> ALKRKIEAAKMPKDAREKTEAELQKLKMMSPMSAEATVVRGYIDWMLQVPWNSRSKVKKDLVKAQEVLDTDHYGLERVKDRILEYLAVQSRVSKIKGPILCLVGPPGVGKTSLGQSIAKATGRQYVRMALGGVRDEAEIRGHRRTYIGSMPGKLIQKMAKVGVKNPLFLLDQIDKMASDMRGDPASALLEVLDPEQNVAFNDHYLEVDYDLSDVMFVATSNSMNIPAPLLDRMEVIRLSGYTEDEKLNIAKQHLLPKQFERNAIKKGELTIDDSAIMSIIRYYTREAGVRSLEREISKLCRKAVKNLLMDKTVKHIEINGDNLKDFLGVQKVDYGRADTENRVGQVTGLAWTEVGGDLLTIETACVPGKGKLTYTGSLGEVMQESIQAALTVVRARADKLGINPDFYEKRDIHVHVPEGATPKDGPSAGIAMCTALVSCLTGNPVRADVAMTGEITLRGLVLPI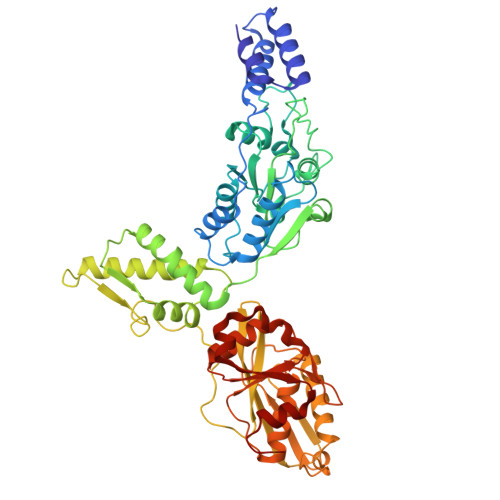GGLKEKLLAAHRGGIKVVLIPDDNKRDLEEIPDNVIADLEIHPVKRIDDVLAIALEHPAF>HPRPLPAGKHAHRQSLETIPEVAELYHCIYK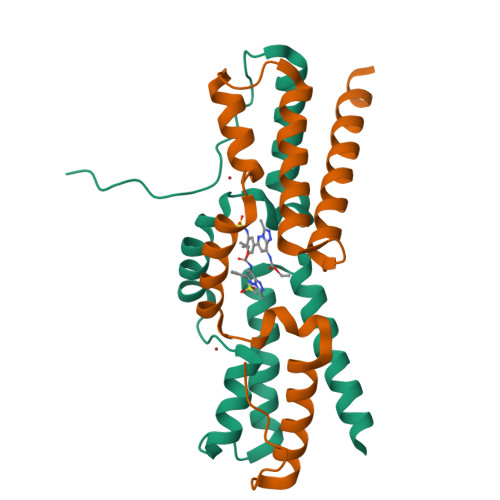LYNEEESSVWFREPVNALAQEIFTYYDVVKSPMSLRHILDNIVKGDTYSTALQVMEDVELIWKNCITFNGANSLLATEAGKCRSALDRIRRAYQDDQRITVEEAE[2x]> DEPRILEAPAPDARRVYVNDPAHFAAVTQQFVIDGEAGRVIGMIDGGFLPNPVVADDGSFIAHASTVFSRIARGERTDYVEVFDPVTLLPTADIELPDAPRFLVGTYPWMTSLTPDGKTLLFYQFSPAPAVGVVDLEGKAFKRMLDVPDCYHIFPTAPDTFFMHCRDGSLAKVAFGTEGTPEITHTEVFHPEDEFLINHPAYSQKAGRLVWPTYTGKIHQIDLSSGDAKFLPAVEALTEAERADGWRPGGWQQVAYHRALDRIYLLVDQRDEWRHKTASRFVVVLDAKTGERLAKFEMGHE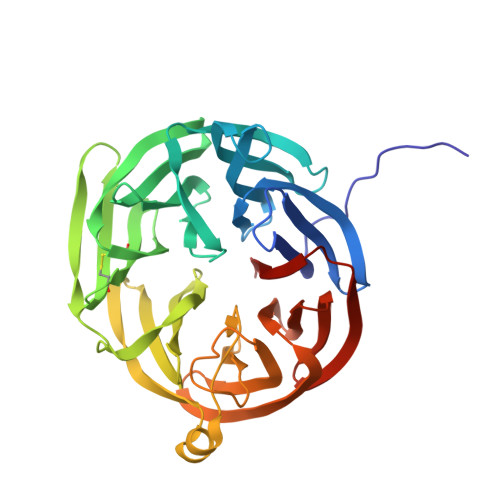IDSINVSQDEKPLLYALSTGDKTLYIHDAESGEELRSVNQLGHGPQVITTADMG>[2x]MIFV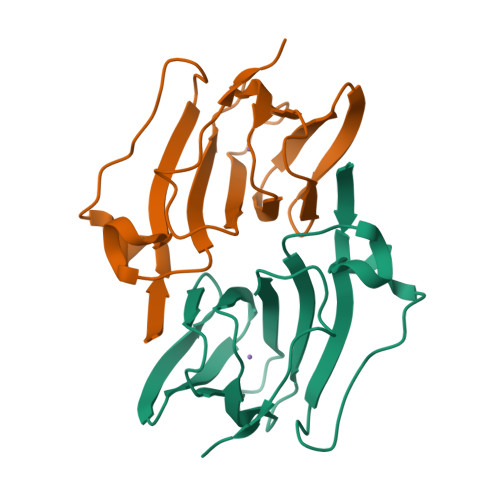KNLASVLSQEWSSTEKYPGVRWKFLIDADFDGSSGLSLGFAEIAPGGDLTLHYHSPAEIAVVTNGKGILNKSGKLETIKKGDVVYIAGNAEHALKNNGKETLEFYWIFPTDRFSEVEYFPAKQKSGHHHHHH> AKMRISPELKKLIEKYRCVKDTEGMSPAKVYKLVGENENLYLKMTDSRY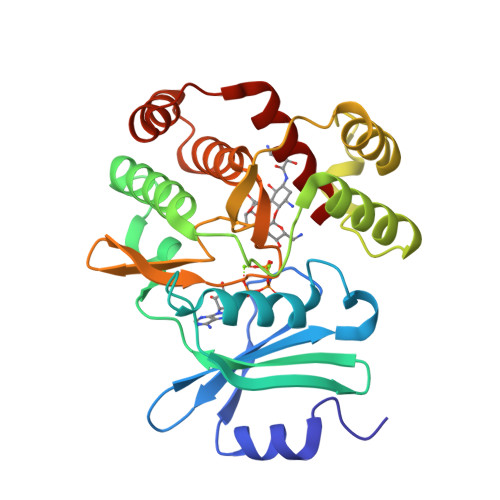KGTTYDVEREKDMMLWLEGKLPVPKVLHFERHDGWSNLLMSEADGVLCSEEYEDEQSPEKIIELYAECIRLFHSIDISDCPYTNSLDSRLAELDYLLNNDLADVDCENWEEDTPFKDPRELYDFLKTEKPEEELVFSHGDLGDSNIFVKDGKVSGFIDLGRSGRADKWYDIAFCVRSIREDIGEEQYVELFFDLLGIKPDWEKIKYYILLDELF> MRCIGISNRDFVEGVSGGSWVDIVLEHGSCVTTMAKNKPTLDFELIETEAKQPATLRKYC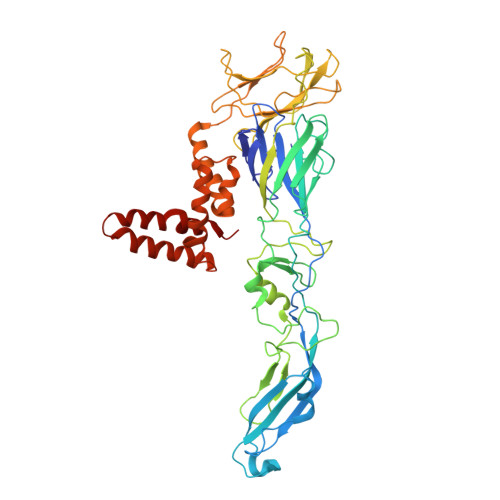IEAKLTNTTTDSRCPTQGEPSLNEEQDKRFVCKHSMVDRGWGNGCGLFGKGGIVTCAMFTCKKNMKGKVVQPENLEYTIVITPHSGEEHAVGNDTGKHGKEIKITPQSSITEAELTGYGTVTMECSPRTGLDFNEMVLLQMENKAWLVHRQWFLDLPLPWLPGADTQGSNWIQKETLVTFKNPHAKKQDVVVLGSQEGAMHTALTGATEIQMSSGNLLFTGHLKCRLRMDKLQLKGMSYSMCTGKFKVVKEIAETQHGTIVIRVQYEGDGSPCKIPFEIMDLEKRHVLGRLITVNPIVTEKDSPVNIEAEPPFGDSYIIIGVEPGQLKLNWFKKGSSIGQMIETTMRGAKRMAILGDTAWDFGSLGGVFTSIGKALHQVFGAIYGAAFSGVSWIMKILIGVIITWIGMNSRSTSLSVSLVLVGVVTLYLGVMVQA>[12x]GAMGIGKSPTGIQGFDELTLGGLPTGRPSLVCGSAGCGKTLFASTFLINGVRDHGEPGVFVTFEERPEDIVNNVASLGFELDKLIEEEKIAIEHIAVDPSEVAEIGDYDLEGLFLRLELAIDTVGAKRVVLDTIESLFSAFSNPAILRAEIRRLFDWLKERGLTTVITAERGDGALTRQGLEEYVSDCVILLDHRVENQISTRRLRIVKYRGTAHGTNEYPFLIDTDGFSVLPVSALGLLHQVHEERIASGVPDLDAMMAGGGFFRGSSILVSGVAGAGKSSLAAHFAAAACARGERAMYFSFEEAADQAVRNMRSLGLDLGRWRDAGLLRFMATRPTFYSLEMHLAVILREVMRFEPSVVVLDPISAFTESGDRLEVQSMLLRIVDFLKNRGITGIFTHLAHSQNEATTDAGLEELMDGWVLMLNREVNGEFNRELYLLKARGMAHSNQVREFLMSDRGISLLPPHLGEGGALTGTARKAEEARLRRAEIERQTELGRLQQQIEQRRRRARAQIEALEAELQAEEIALKALVESESAHERQRLADADTLARSRGNERFADLLMNKGE

Here we investigate the primordial circadian clock in Rhodobacter sphaeroides, which contains only KaiBC, to elucidate its inner workings despite missing KaiA. Using a combination of X-ray crystallography and cryogenic electron microscopy, we find a new dodecameric fold for KaiC, in which two hexamers are held together by a coiled-coil bundle of 12 helices. This interaction is formed by the carboxy-terminal extension of KaiC and serves as an ancient regulatory moiety that is later superseded by KaiA. Our kinetic data identify the difference in the ATP-to-ADP ratio between day and night as the environmental cue that drives the clock.

A coiled-coil register shift between daytime and night-time conformations is connected to phosphorylation sites through a long-range allosteric network that spans over 140 Å. Following phosphorylation, the coiled-coil pairs swap partners by interacting with the other neighbouring chain from the opposite hexamer, which resulted in a register shift that propagated around 115 Å along the entire coiled-coil. In the phosphomimetic state, the register comprised bulkier hydrophobic residues that resulted in a more stable interaction than for the dephosphorylated form. Furthermore, the C-terminal residues of KaiCRS-S413E/S414E interacted with the CII domain of the opposite hexamer, whereas the lack of electron density for the last 30 residues in the wild-type structure indicates more flexibility in the dephosphorylated state. We discovered that these conformational changes in the coiled-coil domain seemed to be coupled through a long-range allosteric network to the phosphorylation sites. The rotameric states of residues Ser413, Ser414, Trp419, Val421, Tyr436, Leu438, Val449 and Arg450 moved concertedly and pointed towards the nucleotide-binding site when the protein was phosphorylated or pointed away in the absence of a phosphate group. We propose that the proximity of the nucleotide to the phosphorylated residue facilitated more efficient phosphoryl transfer.>MPRNFTLFTGQWADLPLEEVCRLARDFGYDGLELACWGDHFEVDKALADPSYVDSRHQLLDKYGLKCWAISNHLVGQAVCDAIIDERHEAILPARIWGDGDAEGVRQRAAAEIKDTARAAARLGVDTVIGFTGSAIWHLVAMFPPAPESMIERGYQDFADRWNPILDVFDAEGVRFAHEVHPSEIAYDYWTTHRALEAVGHRPAFGLNFDPSHFVWQDLDPVGFLWDFRDRIYHVDCKEARKRLDGRNGRLGSHLPWGDPRRGWDFVSAGHGDVPWEDVFRMLRSIDYQGPVSVEW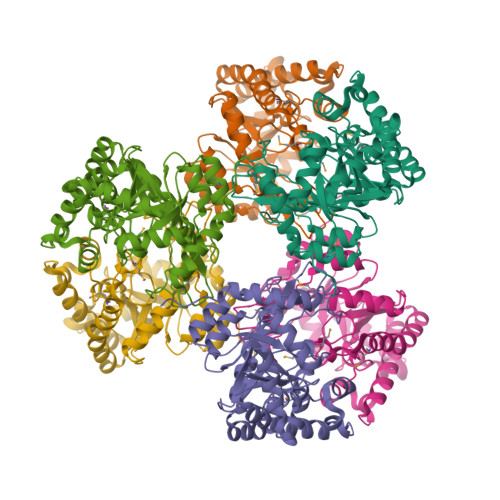EDAGMDRLQGAPEALTRLKAFDFEPPSASFDAAFNSLEHHHHHH[6x]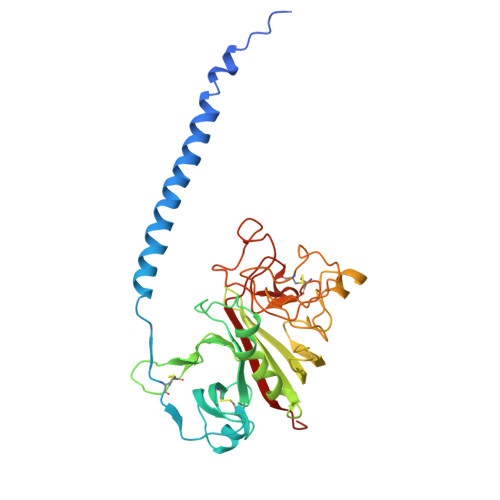> DNENVVNEYSSELEKHQLYIDETVNSNIPTNLRVLRSILENLRSKIQKLESDVSAQMEYCRTPCTVSCNIPVVSGKECEEIIRKGGETSEMYLIQPDSSVKPYRVYCDMNTENGGWTVIQNRQDGSVDFGRKWDPYKQGFGNVATNTDGKNYCGLPGEYWLGNDKISQLTRMGPTELLIEMEDWKGDKVKAHYGGFTVQNEANKYQISVNKYRGTAGNALMDGASQLMGENRTMTIHNGMFFSTYDRDNDGWLTSDPRKQCSKEDGGGWWYNRCHAANPNGRYYWGGQYTWDMAKHGTDDGVVWMNWKGSWYSMRKMSMKIRPFFPQQ Amide Bond Synthetases (ABSs) actively catalyze both the ATP-dependent adenylation of carboxylic acid substrates and their subsequent amidation using an amine nucleophile, both within the active site of the enzyme, enabling the use of only a small excess of the amine partner. In this report, we describe the activity and specificity of an ABS from Streptoalloteichus hindustanus (ShABS), with a broader, complementary substrate spectrum to that of McbA that includes enantioselective behavior toward an expanded range of acid and amine partners in amidation reactions. The requirement for large excesses of amine in these reactions has prompted investigations into the ATP-dependent amide bond synthetase (ABS) class of enzymes, also members of the larger ANL (acyl-CoA synthetase–non-ribosomal peptide synthase–luciferase) family of adenylase enzymes, as these catalyze both the formation of the adenylate and the amidation reaction within one active site of the enzyme and require only one or low equivalents of the amine as a coupling partner. In common with other adenylases, McbA features a larger N-terminal domain coupled to a C-terminal “cap” domain.

Later, an additional structure of ShABS was also obtained from crystallization of the wild-type enzyme in space group P6322 (Data set #3), which had been cocrystallized with the amide product 10a. This ShABS structure (ShABSopen) displayed a rotation, as determined using the Dyndom server, of the cap domain of 81° in the opposite direction to the rotation observed between McbAAd and McbAAm, to expose the active site completely. Although no electron density for a ligand was observed, as the enzyme in these experiments had been complexed with the amide product, we speculate that this conformation may be representative of an exit protein-product complex assumed by ShABS following product release.

> MGYLHRVVEGLKANAGGEALVSADRRLTGAETLEEIHRTARALAAQGLRPGDGVVTLHGNGVEAVVLRIAVQLLGCRYAGLRPVFATREKANFLAEAEAAAFVYQPDMADEAAELLREVPTPRVLSLGPAPLGEDLVALAGAQSAEPVEFTADERAATAVGFTGGTTGRAKGVCRAPFDLEACLDASLTIFGEGPWRFLVCIPIADLGGEMAEWTLAAGGTVVLREDFEPADILATIGAERTTHVFCAPGWVYQLAEHPALADADLSSLTQIPYGGAPSTPARIADALEKLGRPLLVHCYGSQEGGWMTWLSAEDHVRADRYLLNSVGKALPGTEIAIRDQDGADLPVGTVGEVCVRSTMLMRGYWRLPELTAKTVRDGWLHTGDLGRLDTEGYLYLVDRAKDVIIVEAYNVYSQEVEHVLTGHPDVRYAAVVGVPDHDTTEAVYAAVVPAEGVGEIDVDELRALVRTTLGPVHEPKHLDVVDTIPTTPRGKPDKSALRTRWRAAQRA(2S)-amino[(5S)-4,5-dihydro-1,2-oxazol-5-yl]acetic acid | C5 H8 N2 O3 | 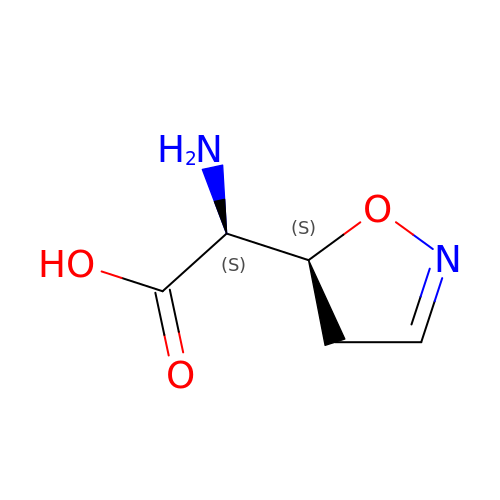CHVHVQLSTPEEOL-IMJSIDKUSA-N>MISKGFSTQTERINILKAQILNAKPCVESERAILITESFKQTEGQPAILRRALALKHILENIPITIRDQELIVGSLTKEPRSSQVFPEFSNKWLQDELDRLNKRTGDAFQISEESKEKLKDVFEYWNGKTTSELATSYMTEETREAVNCDVFTVGNYYYNGV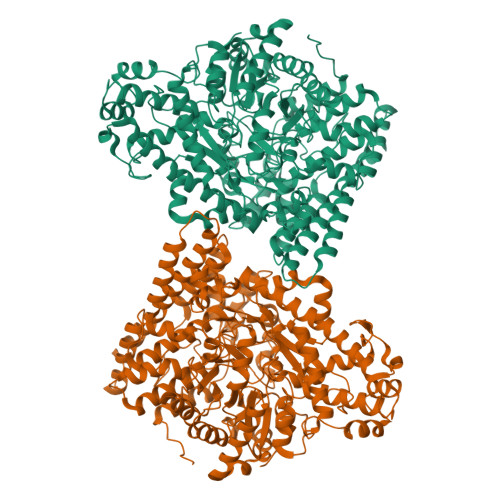GHVSVDYGKVLRVGFNGIINEAKEQLEKNRSIDPDFIKKEKFLNSVIISCEAAITYVNRYAKKAKEIADNTSDAKRKAELNEIAKICSKVSGEGAKSFYEACQLFWFIHAIINIESNGHSISPARFDQYMYPYYENDKNITDKFAQELIDCIWIKLNDINKVRDEISTKHFGGYPMYQNLIVGGQNSEGKDATNKVSYMALEAAVHVKLPQPSLSVRIWNKTPDEFLLRAAELTREGLGLPAYYNDEVIIPALVSRGLTLEDARDYGIIGCVEPQKPGKTEGWHDSAFFNLARIVELTINSGFDKNKQIGPKTQNFEEMKSFDEFMKAYKAQMEYFVKHMCCADNCIDIAHAERAPLPFLSSMVDNCIGKGKSLQDGGAEYNFSGPQGVGVANIGDSLVAVKKIVFDENKITPSELKKTLNNDFKNSEEIQALLKNAPKFGNDIDEVDNLAREGALVYCREVNKYTNPRGGNFQPGLYPSSINVYFGSLTGATPDGRKSGQPLADGVSPSRGCDVSGPTAACNSVSKLDHFIASNGTLFNQKFHPSALKGDNGLMNLSSLIRSYFDQKGFHVQFNVIDKKILLAAQKNPEKYQDLIVRVAGYSAQFISLDKSIQNDIIARTEHVM[2x]>[3x]HHHHHHMEKKLSDAQV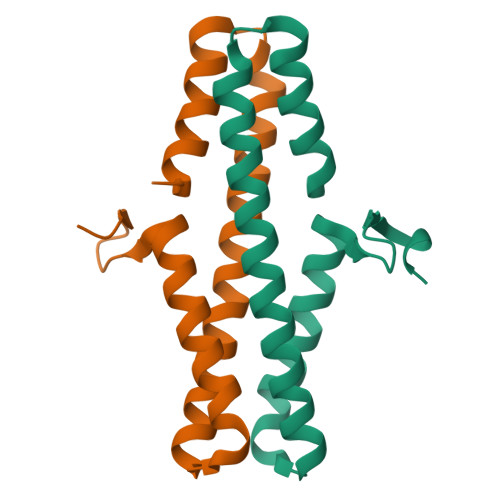ALVAAWRKYPDLRESLEEAASILSLIVFQAETLSDQANELANYIRRQGLEEAEGACRNIDIMRAKWVEVCGEVNQHGIRVYGDAIDRDVD> GSHMTQFEGFTNLYQVSKTLRFELIPQGKTLKHIQEQGFIEEDKARNDHYKELKPIIDRIYKTYADQCLQLVQLDWENLSAAIDSYRKEKTEETRNALIEEQATYRNAIHDYFIGRTDNLTDAINKRHAEIYKGLFKAELFNGKVLKQLGTVTTTEHENALLRSFDKFTTYFSGFYENRKNVFSAEDISTAIPHRIVQDNFPKFKENCHIFTRLITAVPSLREHFENVKKAIGIFVSTSIEEVFSFPFYNQLLTQTQIDLYNQLLGGISREAGTEKIKGLNEVLNLAIQKNDETAHIIASLPHRFIPLFKQILSDRNTLSFILEEFKSDEEVIQSFCKYKTLLRNENVLETAEALFNELNSIDLTHIFISHKKLETISSALCDHWDTLRNALYERRISELTGKITKSAKEKVQRSLKHEDINLQEIISAAGKELSEAFKQKTSEILSHAHAALDQPLPTTLKKQEEKEILKSQLDSLLGLYHLLDWFAVDESNEVDPEFSARLTGIKLEMEPSLSFYNKARNYATKKPYSVEKFKLNFQMPTLASGWDVNKEKNNGAILFVKNGLYYLGIMPKQKGRYKALSFEPTEKTSEGFDKMYYDYFPDAAKMIPKCSTQLKAVTAHFQTHTTPILLSNNFIEPLEITKEIYDLNNPEKEPKKFQTAYAKKTGDQKGYREALCKWIDFTRDFLSKYTKTTSIDLSSLRPSSQYKDLGEYYAELNPLLYHISFQRIAEKEIMDAVETGKLYLFQIYNKDFAKGHHGKPNLHTLYWTGLFSPENLAKTSIKLNGQAELFYRPKSRMKRMAHRLGEKMLNKKLKDQKTPIPDTLYQELYDYVNHRLSHDLSDEARALLPNVITKEVSHEIIKDRRFTSDKFFFHVPITLNYQAANSPSKFNQRVNAYLKEHPETPIIGIDRGERNLIYITVIDSTGKILEQRSLNTIQQFDYQKKLDNREKERVAARQAWSVVGTIKDLKQGYLSQVIHEIVDLMIHYQAVVVLENLNFGFKSKRTGIAEKAVYQQFEKMLIDKLNCLVLKDYPAEKVGGVLNPYQLTDQFTSFAKMGTQSGFLFYVPAPYTSKIDPLTGFVDPFVWKTIKNHESRKHFLEGFDFLHYDVKTGDFILHFKMNRNLSFQRGLPGFMPAWDIVFEKNETQFDAKGTPFIAGKRIVPVIENHRFTGRYRDLYPANELIAL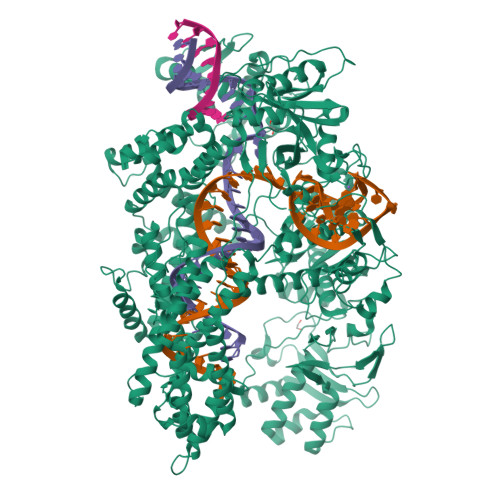LEEKGIVFRDGSNILPKLLENDDSHAIDTMVALIRSVLQMRNSNAATGEDYINSPVRDLNGVCFDSRFQNPEWPMDADANGAYHIALKGQLLLNHLKESKDLKLQNGISNQDWLAYIQELRN(2R,3S,4S,5R,6R)-2-(aminomethyl)-6-[(1R,2S,3S,4R,6S)-4,6-bis(azanyl)-3-[(2S,3R,4S,5S,6R)-6-(hydroxymethyl)-3,4,5-tris(oxidanyl)oxan-2-yl]oxy-2-oxidanyl-cyclohexyl]oxy-oxane-3,4,5-triol 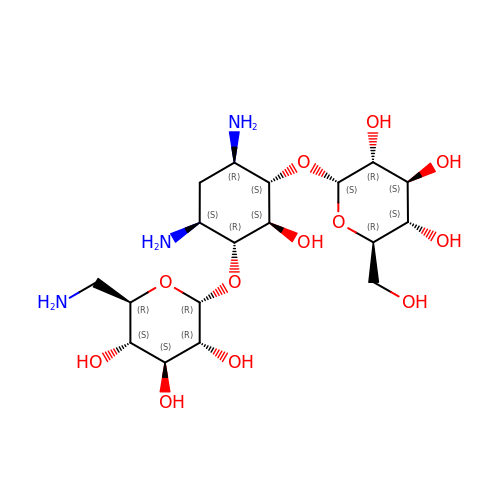| C18 H35 N3 O12 | NZCOZAMBHLSNDW-HNDNCJINSA-N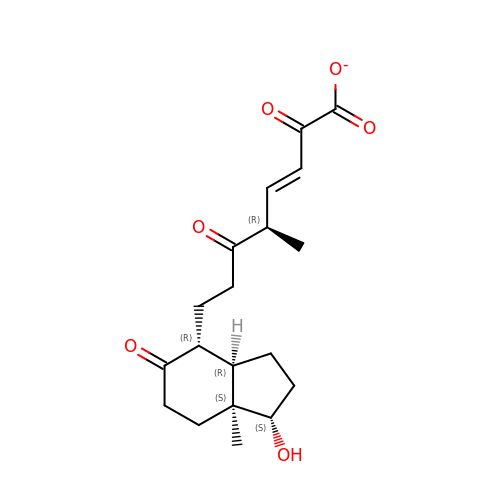(3E,5R)-8-[(1S,3AR,4R,7AS)-1-HYDROXY-7A-METHYL-5-OXOOCTAHYDRO-1H-INDEN-4-YL]-5-METHYL-2,6-DIOXOOCT-3-ENOATE | C19 H25 O6 | PAPYZGVUTPWUFW-WDRCEGBMSA-M> SMNKLYIGNLSDH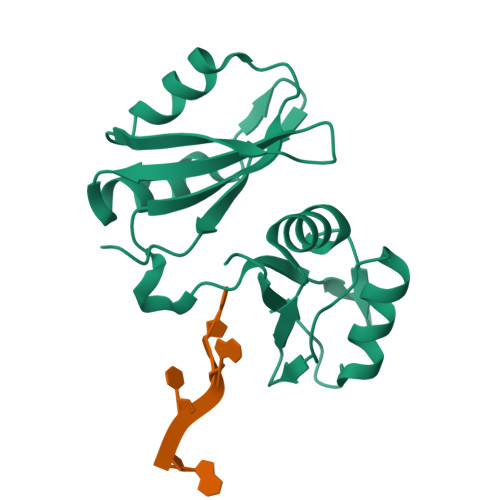AGPADLESVFKDAKIPVAGPFLVKTGYAFVDCPDEGWALKAIEALSGKMELHGKPMEVEHSVPKRQRIRKLQIRNIPPHLQWEVLDSLLVQYGVVESCEQVNTDSETAVVNVTYSSKDQARQALDKLNGFQLENFTLKVAYIPDETAAQ> GGUG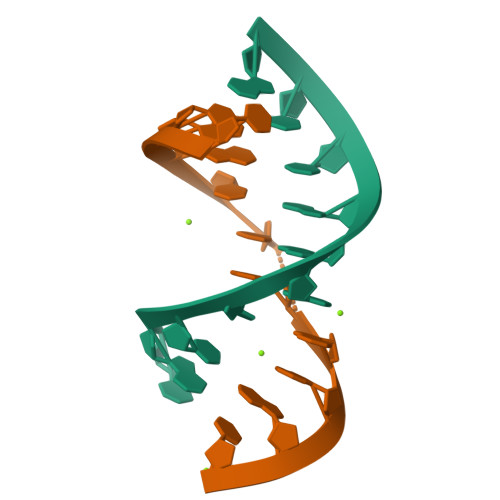AGGCUG;> CCAGUCGGAAC>GMLDNAIPQGFEDAVELRRKNRETVVKYMNTKGQDRLRRHELFVEDGCGGLWTTDTGSPIVIRGKDKLAEHAVWSLKCFPDWEWYNIKVFETDDPNHFWVECDGHGKILFPGYPEGYYENHFLHSFELDDGKIKRNREFMNVFQQLRALSIPVPQIKRE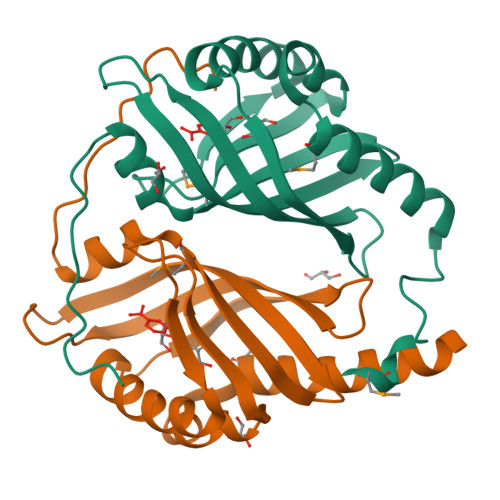GIPT[2x]ORP1L, a long ORP1 variant (hereafter referred to as ORP1), is specifically localized to the contact sites between the late endosomes/lysosomes (LELs) and the ER and implicated in non-vesicular sterol transport. The N-terminal ANK domain targets ORP1 to the LELs via interaction with the Rab7 anchored to the endosomal membrane.. Rab7 functions as a key regulator in maturation of endosomes and autophagosomes, directing the trafficking of cargos along microtubules, and in the fusion step with lysosomes, through different protein-protein interaction cascades. Here we characterized the structural and molecular details of the human ORP1 ANK–Rab7 interaction by determination of the crystal structure and biochemical analysis of the interaction.

The asymmetric unit of the crystal contained two heterodimers of the ORP1–Rab7 complex. The bound GTP and Mg2+ ion in Rab7 were clearly visible in the 2.1 Å electron density maps. In the crystal structure, the GTP-bound Rab7 has a closed conformation of switch regions. The human ORP1 ANK is composed of four helix-turn-helix repeats connected by a long or tight β-hairpin loop. ORP1 ANK binds to Rab7 using the concave surface composed of the inner helices of ANK repeats and the first β-hairpin loop. The helix α3 and the α3-β5 loop of Rab7 compose the ANK binding site. The switch I and switch II regions which undergo conformational changes upon GTP or GDP binding are away from the interface, indicating the independence of ORP1–Rab7 interaction from the nucleotide binding. Several basic residues such as Arg14, Arg87, and Arg93 of ORP1 make hydrogen bonds with Asp104, Ser111, and Glu116 of Rab7. The bulky hydrophobic residues including Trp49, Phe50, Tyr57, and Phe58 from ORP1 make hydrophobic interaction with the residues on the helix α3 and the α3-β5 loop of Rab7. In the crystal of human ORP1-Rab7, the truncated switch II region with (Δ73) composes the tight crystal lattice interaction, indicating that the surface entropy reduction by L73Δ was critical for crystallization.

>[2x]GSAMGSTSRKKVLLKVIILGDSGVGKTSLMNQYVNKKFSNQYKATIGADFLTKEVMVDDRLVTMQIWDTAGLERFQSGVAFYRGADCCVLVFDVTAPNTFKTLDSWRDEFLIQASPRDPENFPFVVLGNKIDLENRQVATKRAQAWCYSKNNIPYFETSAKEAINVEQAFQTIARNALKQETEVELYNEFPEPIKLDKN;>[2x]GSAMGSAEQQLLHHARNGNAEEVRQLLETMARNEVIADINCKGRSKSNLGWTPLHLACYFGHRQVVQDLLKAGAEVNVLNDMGDTPLHRAAFTGRKELVMLLLEYNADTTIVNGSGQTAKEVTHAEEIRSMLEAVERTQQRKLEELLLAAAREG>QGPSSPMDSSRRQYQEKYKQVEQYMSFHKLPADMRQKIHDYYEHRYQGKIFDEENILSELNDPLREEIVNFNCRKLVATMPLFANADPNFVTAMLSKLRFEVFQPGDYIIREGAVGKKMYFIQHGVAG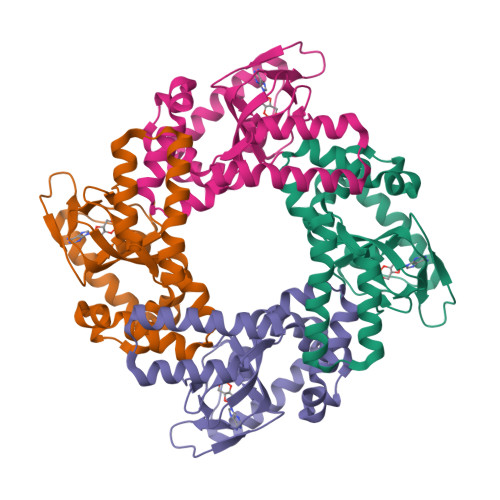VITKSSKEMKLTDGSYFGEICLLTKGRRTASVRADTYCRLYSLSVDNFNEVLEEYPMMRRAFETVAIDRLDRIGKKNSILLQ[2x]Coat protein 1 (COPI) coated vesicles function in retrograde trafficking between the Golgi apparatus and the Endoplasmic Reticulum (ER), and between the Golgi cisternae in both retrograde and anterograde directions. Coatomer (the COPI complex) is a heteroheptameric protein complex, consisting of α, β, β’, γ, δ, ε and ζ subunits. Arf1-GTP recruits the protein complex coatomer from the cytoplasm and anchors it at the membrane. Polymerization of coatomer at the membrane assembles the COPI coat, which recruits cargo molecules and membrane machinery to the assembly site.

Crystal structures were available for the majority of the components of the COPI coat, but not for the βδ-COP subcomplex. As a first step towards a complete structural model, we expressed and crystallized a complex containing β-COP19-391 and δ-COP1-175 from C. thermophilum (Ct), from which we obtained a molecular model of βδ-COP comprising residues 20–390 of β-COP (‘trunk region’) and residues 2–150 of δ-COP. The overall architecture of βδ-COP is similar to that of the homologous γζ-COP. β-COP(20-390) is a curved HEAT-repeat type α-solenoid consisting of 20 consecutive α-helices. The right-handed super-helical arch of β-COP wraps around the δ-subunit. The structural model of δ-COP comprises a longin domain followed by a β-turn (117-122), and two helices a (127-135) and b (139-150), which are part of the linker region connecting the longin domain and the μ-Homology Domain (MHD). The stretch of residues between helix a and amphipathic helix b traverses the β-COP α-solenoid in the vicinity of helix 7. Helix b, including isoleucine residues 143, 146 and 147, projects away from the α-solenoid where it would be accessible for binding partners. Helix a and the first part of helix b are present in our x-ray structure. While no electron density was visible for residues 151–175 of δ-COP in the x-ray structure, our cryoEM map of the COPI coat has clear density corresponding to a longer helix, and we modeled residues 139–165 of the predicted helix b into our density. The sequence identity between the βδ-COP from Chaetomium thermophilum used for crystallography and Mus musculus used for subtomogram averaging is 53%.

> TPTLQELKTQLEKGNDETKIETMKRILTIMLNGDPLHGLLMHIIRFVMPSKSKPLKKLLYFYYEICPKLDSQGKLKQEFILVCNGIRNDLQHPNEYIRGNTLRFLCKLREPELLEPLLSSVRACLEHRHAYVRKNAVFAVASIYQHAPSLIPDAADLIATFLEGESDPTCKRNGFAALSSISHDKALSYLGTVFEGIPNAEELLQLVEIEFIRKDALHNPQNKPRYLRLIFDLLEANTSTVVYEAASSLTALTNNPVAVKAAAGKFIELAIKEADNNVKLIVLDRVDQLRQKNEGILDDLIMEILRVLSSPDIDVRRKALEIALEMVSSKNVEEVVLLLKKELSKTVEQEYEKNSEYRQLLIHSIHQCAVKFS;> MVVLAASICTRGGKAVLARAFHDIKRSRVEALLASFPKAANSGTQHTTVEQDNVRFVYQPLDELYMVLITNKQSNILQDIDTLHLFAQVVTNTCRTLEEREILRNAYELISAFDEIINLGYRENLTINQIKTFLEMESHEERIQEIIARNKELEATEERKRKAKQLEMQRKEASR> MSQEQGKIY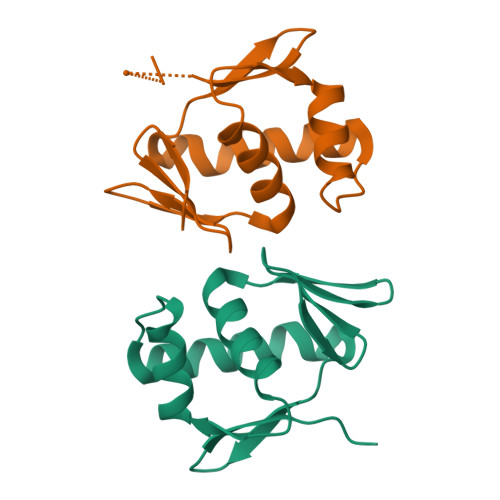IVEDDMTIVSLLKDHLSASYHVSSVSNFRDVKQEIIAFQPDLILMDITLPYFNGFYWTAELRKFLTIPIIFISSSNDEMDMVMALNMGGDDFISKPFSLAVLDAKLTAILRRSQQFIQQELTFGGFTLTREGLLSSQDKEVILSPTENKILSILLMHPKQVVSKESLLEKLWENDSFIDQNTLNVNMTRLRKKIVPIGFDYIHTVRGVGYLLQDPNSSSVDKLAAALEHHHHHH;> MSQEQGKIYIVEDDMTIVSLLKDHLSASYHVSSVSNFRDVKQEIIAFQPDLILMDITLPYFNGFYWTAELRKFLTIPIIFISSSNDEMDMVMALNMGGDDFISKPFSLAVLDAKLTAILRRSQQFIQQELTFGGFTLTREGLLSSQDKEVILSPTENKILSILLMHPKQVVSKESLLEKLWENDSFIDQNTLNVNMTRLRKKIVPIGFDYIHTVRGVGYLLQNDPSSSVDKLAAALEHHHHHH A similar cleavage reaction was observed in vitro with other enzymes from diverse organisms, including a snake venom phosphodiesterase (SVP), mammalian ectonucleotide pyrophosphatase/phosphodiesterase 1 (ENPP1), Escherichia coli RppH (EcRppH), and Homo sapiens NudT16 (HsNudT16). In addition, although NudT16 was initially characterized as a nucleolar U8 snoRNA decapping enzyme, it is involved in mRNA decapping and expresses across mouse tissues. Given the versatility in the recognition of substrates with diphosphate bonds, we and others have used some of these Nudix enzymes in vitro for processing ADP-ribosylation to a unique mass tag for site identification by tandem mass spectrometry (MS/MS). In this study, we sought to understand how HsNudT16 binds and hydrolyzes different forms of ADPr using X-ray crystallography.

Observing that His24 came within close proximity to the adenine base, we also designed H24W mutant to improve base stacking. H24W and F61S mutants behave as dimers in solution as shown by the size-exclusion chromatography profile similar to HsNudT16. Contrary to our hypothesis, the structure of the HsNudT16 H24W shows that the indole ring of the tryptophan, instead of improving stacking, protrudes into the adenosine binding site, as demonstrated by structurally aligning with the HsNudT16-ADPr model. H24W mutant had no significant activity towards free ADPr; consequently, the Km was not measured. The lack of enzymatic activity could be explained by the fact that the indole group of the tryptophan occupies the site of the adenosine and sterically hinders ADPr binding. This is compounded with the loss of interaction between the imidazole ring and the oxygen of the β-phosphate. The insignificant demodification activity with H24W mutant with protein-conjugated ADPr as well as its Michaelis-Menten results on hydrolysis of free ADPr could be explained by the position of the tryptophan in the structure, which suggests that H24W occludes the recognition site of the purine. Under the tested conditions, demodification assays of MARylated PARP10CD showed no clear changes between wild-type HsNudT16 and all mutants except H24W, which had minimal hydrolysis activity.

>[4x]MAGARRLELGEALALGSGWRHVCWALLYAPDPGMLFGRIPLRYAILMQMRFDGRLGFPGGFVDTQDRSLEDGLNRELREELGEAAAAFRVERTDYRSSHVGSGPRVVAHFYAKRLTLEELLAVEAGATRAKDHGLEVLGLVRVPLYTLRDGVGGLPTFLENSFIGSAREQLLEALQDLGLLQSGSISGLKIPAHH> AVCGSVWGQNDLAYRCRTCEHDPT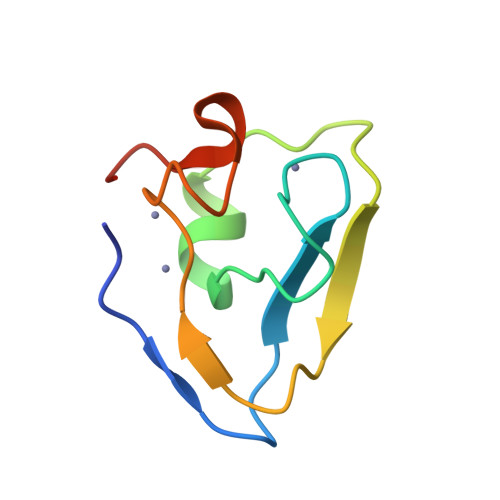CAICVPCFQNGNHKDHDYSIMYTGGGCCDCGDTTAWKREGFCSRHKGA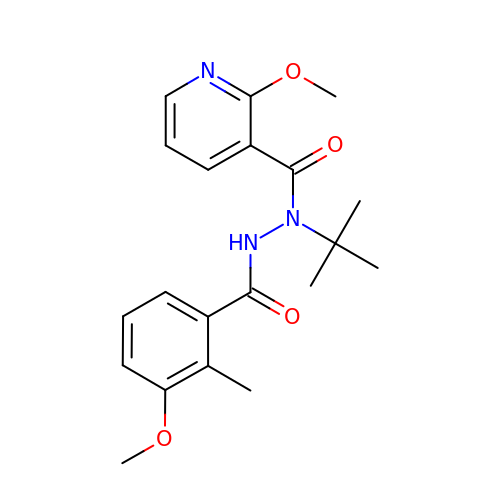~{N}-~{tert}-butyl-2-methoxy-~{N}'-(3-methoxy-2-methyl-phenyl)carbonyl-pyridine-3-carbohydrazide | C20 H25 N3 O4 | IQDJDSKRJNIDTA-UHFFFAOYSA-N> MQAIPMTLRGAEKLREELDFLKSVRRPEIIAAIAEAREHGDLKENAEYHAAREQQGFCE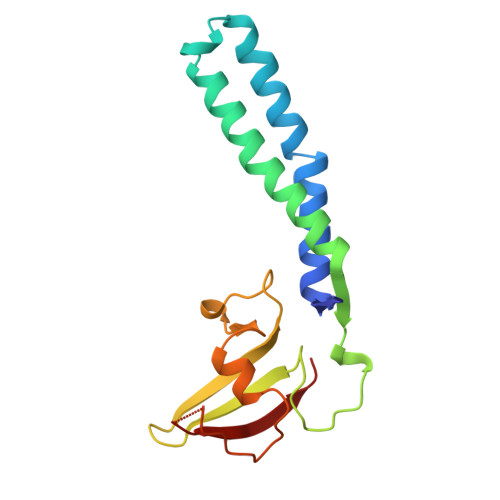GRIKDIEAKLSNAQVIDVTKMPNNGRVIFGATVTVLNLDSDEEQTYRIVGDDEADFKQNLISVNSPIARGLIGKEEDDVVVIKTPGGEVEFEVIKVEYL>[2x]MGSDKIHHHHHHENLYFQGQKKVSILGDSYSTFYGHVSPAANLCWYGVPGEKKENDVT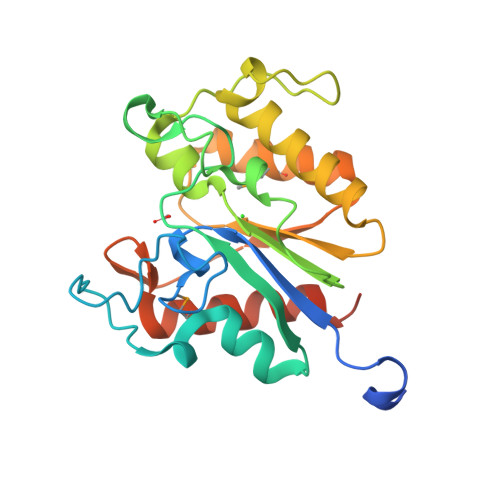KVEETWWYRFIHEHGFQLERNNSYSGSTVCHTGYEKADYSDRSFITRIHNLGTPDIILVFGGTNDSWAGAPIGAYQYDGWTKADLYSFRPAFCYLLASLKQLYPAARIYNITNSELSEEVTDSMDEICRHYGIENIRLHDIDKQWGHPSVQGMQSIDAQVWESVSPILEASVSLPAKN>[4x]GHMRIEVRVDNGR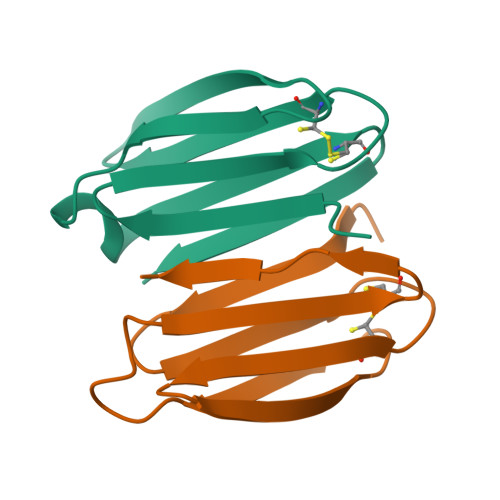VRVRNGTDRPCRVRVTAGGETREYTVNPGTELEVELSPEQQNNAEVEVECGNEKYRFQLG αHBs are oligomers of 5 or more α-helical peptides that assemble into coiled-coil structures with central solvent-accessible channels. We targeted two properties of αHBs: oligomeric state, which directly affects the internal diameter of the channel; and the identities of channel-facing residues, which fine tune this dimension and introduce different chemistries. The αHBs are loaded with an environment sensitive dye (in this case, 1,6-diphenyl-1,3,5-hexatriene, DPH) that binds within the channels and fluoresces. Accordingly, challenging the array with analytes leads to differential displacement of the dye across the array to give a fluorescent fingerprint.

Despite the requirements for aliphatic residues at a and d, up to 40% of these can be changed to other side chains without compromising barrel integrity. We introduced mutations at one or two of these sites to generate four groups of αHB: Group I had entirely hydrophobic interiors, but with different sizes and shapes of channel; Groups II and III had polar uncharged or polar charged residues, respectively, at specific points along the channel; and Group IV had aromatic residues installed in their channels. The eleven Group II peptides comprised: single mutants to Cys, His, Asn, Ser or Thr at d sites; and double mutations to His, Asn, Ser or Thr at consecutive a and d sites. Finally, one third of the designs were crystallized and yielded 12 X-ray crystal structures, all of which were open αHBs with fully accessible channels. Focusing on the small molecules, the αSA signal from the more-polar AAs and CHOs is dominated by the polar and charged Group II and III αHBs.

>XGEIAQALKEIAKALKECAWALKEIAQALKGX[3x]> GPGSMEQPKGINILITGTPGTGKTSMAEMIAAELDGFQHLEVGKLVKENHFYTEYDTELDTHIIEEKDEDRLLDFMEPIMVSRGNHVVDYHSSELFPERWFHMVVVLHTSTEVLFERLTKRQYSEAKRAENMEAEIQCICEEEARDAYEDDIVLVRENDTLEQMAATVEE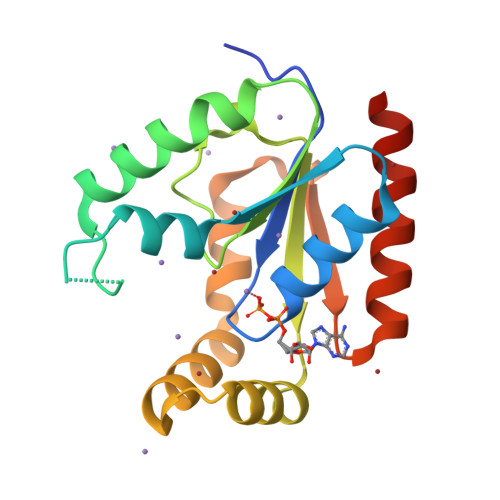IRERVEVLKVERGL> LNTTILTPNGNEDTTADFFLTTMPTDSLSVSTLPLPEVQCFVFNVEYMNCTWNSSSEPQPTNLTLHYWYKNSDNDKVQKCSHYLFSEEITSGCQLQKKEIHLYQTFVVQLQDPREPRRQATQMLKLQNLVIPWAPENLTLHKLSESQLELNWNNRFLNHCLEHLVQYRTDWDHSW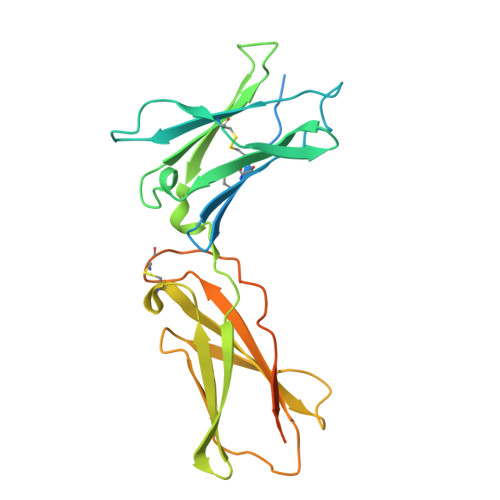TEQSVDYRHKFSLPSVDGQKRYTFRVRSRFNPLCGSAQHWSEWSHPIHWGSNTSKENPFLFALEAGAQDKTHTCPPCPAPELLG>KIFSKCELARKLKSMGMDGFHGYSLANWVCMAEYESNFNTQAF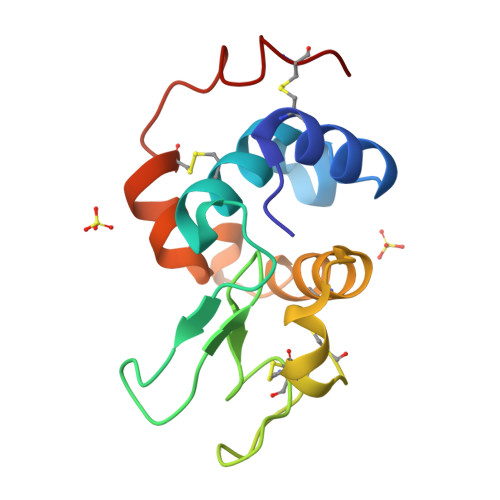NGRNSNGSSDYGIFQLNSKWWCKSNSHSSANACNIMCSKFLDDNIDDDIACAKRVVKDPNGMSAWVAWVKHCKGKDLSKYLASCNL[2x]> DYW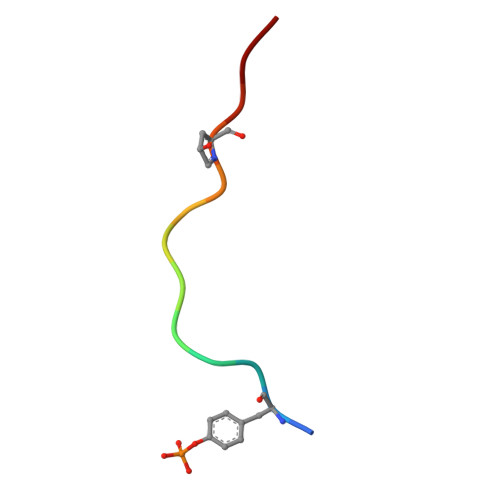KPRHHPPRNN(2~{S})-2-cyano-~{N},~{N}-dimethyl-3-[5-[3-[(1~{S},2~{R})-2-methylcyclohexyl]-3,5,8,10-tetrazatricyclo[7.3.0.0^{2,6}]dodeca-1,4,6,8,11-pentaen-4-yl]furan-2-yl]propanamide 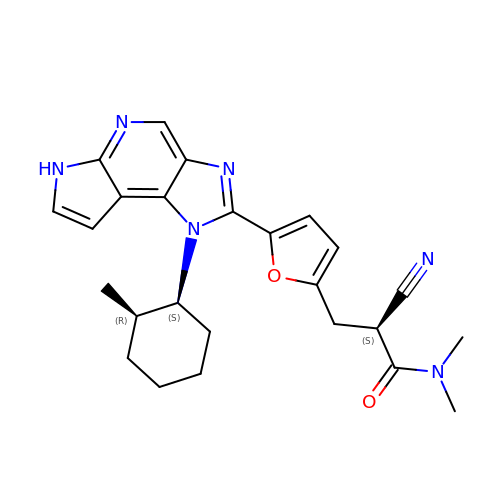| C25 H28 N6 O2 | AMJNKQADUVRGCR-GUXCAODWSA-N(3aS,8S,9aS)-2-acetyl-10-methyl-2,3,6,8,9,9a-hexahydro-3a,8-epiminocyclohepta[1,2-c:4,5-c']dipyrrol-4(1H)-one 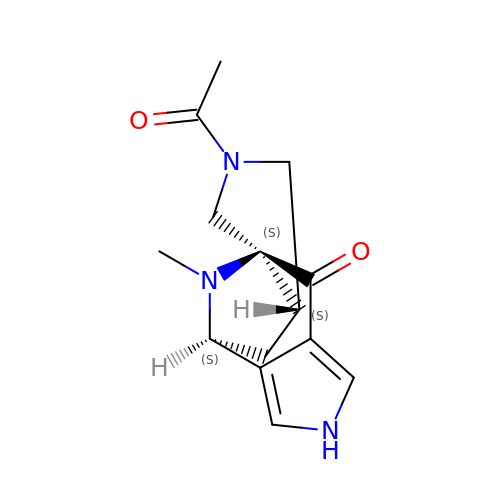| C14 H17 N3 O2 | CPZLROCUKBXZER-DUFXMDAXSA-N> MEDGKRLRIGITLHPYYSYVSNIVGDKAEVVPLIPAGFNPHAYEPRAEDIKRIGTLDVVVLNGVGHDDFAERMIASSEKPGIPVIEANAKVPLLAATGMAARGAGKVVNPHTFLSISASITQVNTIARELGKLDPANAKAYTRNARAYAKRLRALRADALARLNKAPAADFRVATIHGAYDYLLREFGLEVTAVVEPAHGIEPSPSQLKKTID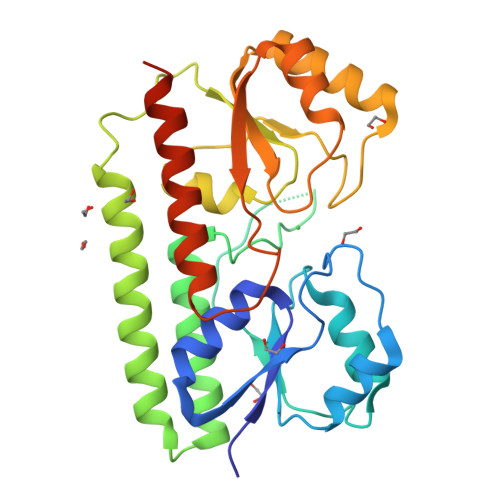QLKALDVKVIFSEIDFPSTYVETIQRESGVKLYSLSHISYGDYSAGKYEEEMARNLDTVVRAIQESGAEILYFQSHHHHHH In this study, by means of glycan microarray screening, NMR, surface plasmon resonance (SPR), and cell binding assays, we show that FA, which is the predominant glycolipid in ovine erythrocytes, serves as a cellular attachment receptor for the VP1 of a polyomavirus originally identified in sheep. This designated sheep polyomavirus (ShPyV) is a member of a non-enveloped, double-stranded DNA virus family with icosahedral capsids, scaffolded by the major capsid protein VP1. Here, glycan array screening shows that the major capsid protein VP1 of sheep polyomavirus (ShPyV) binds to the Forssman glycolipid, an antigen of many vertebrates and a potential tumor marker in humans. We show that the Forssman antigen serves as a cellular attachment receptor for the major capsid protein VP1 of ShPyV. Thus, our studies present the first example of a polyomavirus VP1 protein interacting with a non-sialyl neutral glycan, complementing the principles of how polyomaviruses recognize their targets.

We also solved the crystal structure of VP1 in complex with the FA glycan precursor, globo-*N*-tetraose, which reveals negligible binding only. We therefore conclude that the terminal GalNAcα1-3GalNAc disaccharide is essential for the high affinity of the ShPyV VP1-FP complex. A dominance of the terminal GalNAcα1-3GalNAcβ Forssman disaccharide is apparent as the VP1 did not give binding signals with globoside glycolipid (P-antigen, position 25, [Table tbl1]), the precursor of the Forssman glycolipid which lacks the terminal α-linked GalNAc residue.

>GSHMGGIEVLAVRTGPDSITEIEAYLNPRMGQPQNEDFYGFSDNVTVSDDFGSDAPPWKQFPCYSTARISLPMLNQDMTSDTILMWEAISCRTEVMGVNMLTNVHSAQKRVYENDREGTGIGVEGMGYHMFAIGGEPLELQFMVFNHRATYPAEATVIKNPGASSQVFDPNLKGTLTADGVFPVEAWGPDPFKNENTRYFGQYTGGTQTPPVLTFTNTQTTILLDENGVGPLCKGDGLFLSCADIVGFFTQHNKKMSFRGLPRYFRVTLRKRVVKN[10x]> GGGGUGUGCCCGGCAUGGGUGCAGUCUAUAGGGUGAGAGUCCCGAACUGUGAAGGCAGAAGUAACAGUUAGCCUAACGCAAGGGUGUCCGUGGCGACAUGGAAUCUGAAGGAAGCGGACGGCAAACCUUCGGUCUGAGGAACACGAACUUCAUAUGAGGCUAGG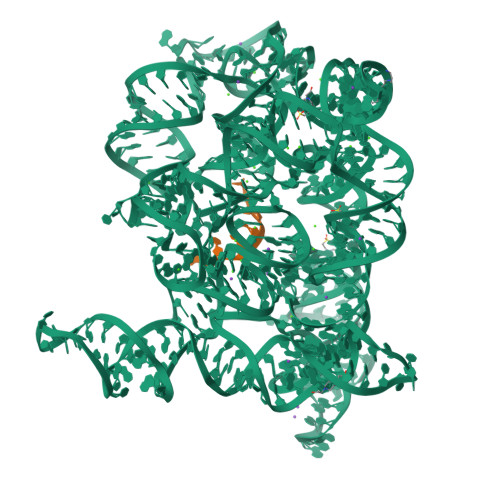UAUCAAUGGAUGAGUUUGCAUAACAAAACAAAGUCCUUUCUGCCAAAGUUGGUACAGAGUAAAUGAAGCAGAUUGAUGAAGGGAAAGACUGCAUUCUUACCCGGGGAGGUCUGGAAACAGAAGUCAGCAGAAGUCAUAGUACCCUGUUCGCAGGGGAAGGACGGAACAAGUAUGGCGUUCGCGCCUAAGCUUGAACCGCCGUAUACCGAACGGUACGUACGGUGGUGUG;> CGAUUUAUUA The ABC transporter McjD exports the antibacterial peptide MccJ25 in Escherichia coli. Four genes are required for the biosynthesis and export of MccJ25 (Duquesne et al, 2007b): mcjA encodes the linear precursor of MccJ25; mcjB and mcjC encode enzymes involved in the post‐translational modification of McjA to the lasso structure; and mcjD encodes an ABC exporter that is required for both MccJ25 secretion and self‐immunity of the producing strain towards MccJ25 (Choudhury et al, 2014). We have previously functionally characterized and determined the high‐resolution structure of McjD from Escherichia coli (Choudhury et al, 2014). Its core architecture is composed of a dimeric transmembrane domain (TMD) of 12 transmembrane (TM) helices, which forms the translocation pathway across the membrane bilayer and contains the ligand binding site, and a dimeric nucleotide binding domain (NBD) where ATP binds and is hydrolysed. In this study, we have determined its structure in a novel conformation, apo inward‐occluded and a new nucleotide‐bound state, high‐energy outward‐occluded intermediate state, with a defined ligand binding cavity.

The McjD‐apo structure was also determined by molecular replacement using the McjD‐AMPPNP structure but only after splitting the McjD monomer into two domains, TMD and NBD. Inspection of the NBDs did not reveal any electron density for nucleotides that may have been co‐purified with McjD. A striking difference between McjD‐apo and other apo ABC exporters, such as MsbA (Ward et al, 2007) and PglK (Perez et al, 2015), is that its TMD is in an occluded conformation, similar to the McjD‐AMPPNP structure, whereas the NBDs have disengaged in the absence of nucleotides. This conformation is called here apo inward‐occluded. Inward‐facing ABC exporters display domain intertwining of TMs 1–3 and 6 from one subunit and TMs 4–5 from the opposite subunit, which results in opening of the TMD to the cytoplasmic side of the inner membrane (Ward et al, 2007; Perez et al, 2015). In the inward‐occluded McjD, TMs 3–5 from one subunit have moved towards the equivalent TMs of the opposite subunit, resulting in the loss of intertwining and occlusion of the cytoplasmic opening (Figs 2B and EV2). The McjD‐apo structure can be superimposed with the McjD‐AMPPNP structure with an rmsd of 2.1 Å over 569 Cα atoms; their TMDs can be superimposed with an rmsd of 0.7 Å over 290 Cα atoms. The NBDs of the McjD‐apo have separated by 7.9 Å (measured between S509 and S509’) relative to the McjD‐AMPPNP structure, a distance much shorter compared to MsbA‐apo with a distance of 35 Å (Ward et al, 2007). The NBDs have moved in a “scissors‐like” motion similar to the transition between inward and outward‐open MsbA. We designed the A122C mutant at the beginning of TM3 on the cytoplasmic side of McjD, with a Cα‐Cα′ distance of 7.3 Å.

> MERKQKNSLFNYIYSLMDVRGKFLFFSMLFITSLSSIIISISPLILAKITDLLSGSLSNFSYEYLVLLACLYMFCVISNKASVFLFMILQSSLRINMQKKMSLKYLRELYNENITNLSKNNAGYTTQSLNQASNDIYILVRNVSQNILSPVIQLISTIVVVLSTKDWFSAGVFFLYILVFVIFNTRLTGSLASLRKHSMDITLNSYSLLSDTVDNMIAAKKNNALRLISERYEDALTQENNAQKKYWLLSSKVLLLNSLLAVILFGSVFIYNILGVLNGVVSIGHFIMITSYIILLSTPVENIGALLSEIRQSMSSLAGFIQRHAENKATSPSIPFLNMERKLNLSIRELSFSYSDDKKILNSVSLDLFTGKMYSLTGPSGSGKSTLVKIISGYYKNYFGDIYLNDISLRNISDEDLNDAIYYLTQDDYIFMDTLRFNLRLANYDASENEIFKVLKLANLSVVNNEPVSLDTHLINRGNNYSGGQKQRISLARLFLRKPAIIIIDEATSALDYINESEILSSIRTHFPDALIINISHRINLLECSDCVYVLNEGNIVASGHFRDLMVSNEYISGLASVTE> GSPTFKSAVKALFDYKAQREDELTFTKSAIIQNVEKQDGGW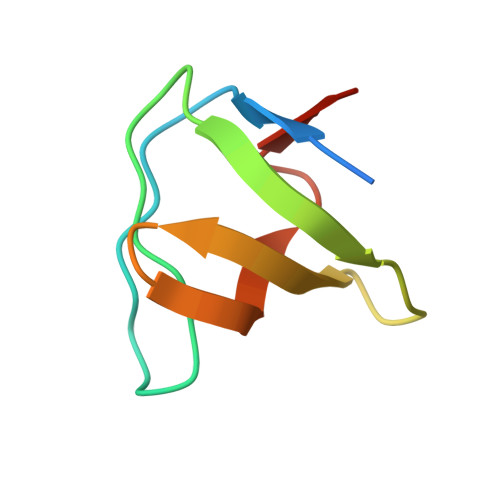WRGDYGGKKQLWFPSNYVEEMIN> MADG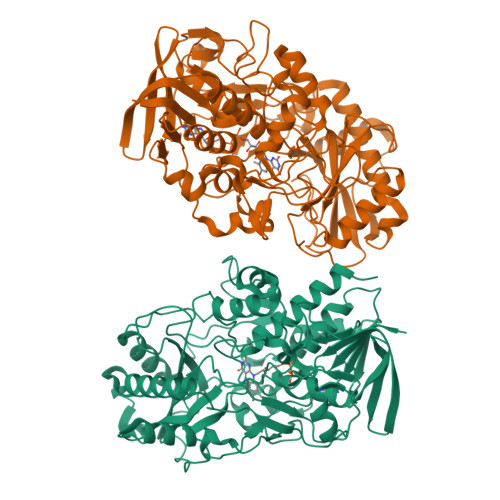VRMTRAKVEHAPNCDIVIVGGGSAGSLLAARLSEDPDSRVLLIEAGEEPTDPDIWNPAAWPALQGRSYDWDYRTEAQAGTAGRAHHWARGRLIGGSSCLHAMGYMRGHPSDFQAWVDASGDRRWGWDELLPVFQAIEDHPLGGDGIHGKGGPLPIHLPADEVSPLARAFIEAGASLGLPRLEGHNSGEMIGVTPNSLNIRDGRRVTAADAWLTKAVRGRKNLTILTGSRVRRLKLEGNQVRSLEVVGRQGSAEVFADQIVLCAGALESPALLMRSGIGPHDVLDAAGVGCLIDMPDIGRNLQDHLLGAGNLYAARKPVPPSRLQHSESMAYMRADSFTAAGQPEIVVGCGVAPIVSESFPAPAAGSAYSLLFGITHPTSRGSVRISGPELGDRLIIDPAYLQTGRDRERFRRALEASRTIGHRDELAGWRERELLPGTPNSAAEMDDFIARSVITHHHPCGTCRMGKDPDAVVDANLRLKALDNLFVVDASIMPNLTAGPIHAAVLAIAETFARQYHHHHHH>[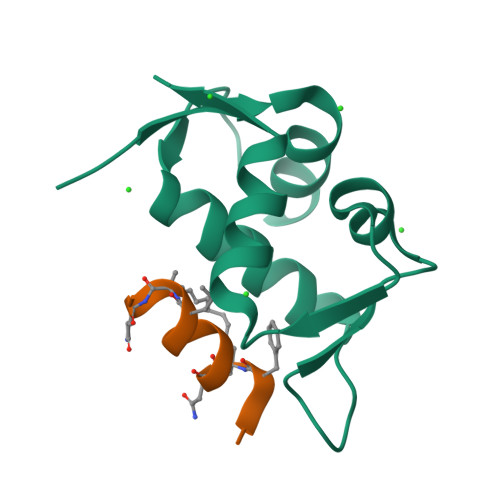2x]MQETLVRPKPLLLKLLKSVGAQKDTYTMKEVLFYLGQYIMTKRLYDEKQQHIVYCSNDLLGDLFGVPSFSVKEHRKIYTMIYRNLVVV;>QSQQTFXNLWRLLLQN[2x]>MCPTLNNIVSSLQRNGIFINSLIAALTIGGQQLFSSSTFSCPCQVGKNFYYGSAFLVIPALILLVAGFALRSQMWTITGEYCCSCAPPYRRISPLECKLACLRFFSITGRAVIAPLTWLAVTLLTGTYYECAASEFASVDHYPMFDNVSASKREEILAGFPCCRSAPSDVILVRDEIALLHRYQSQMLGWILITLAT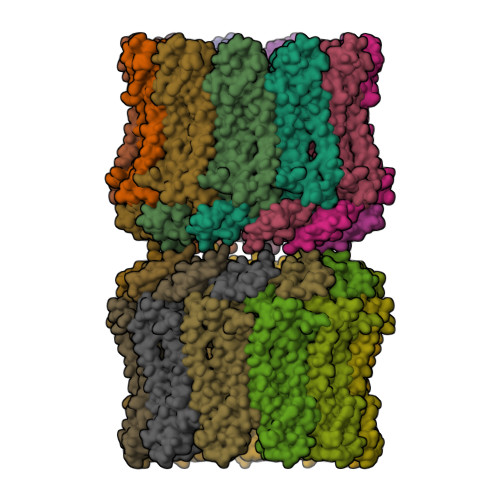IAALVSCCVAKCCSPLTSLQHCYWTSHLQNERELFEQAAEQHSRLLMMHRIKKLFGFIPGSEDVKHIRIPSCQDWKDISVPTLLCMGDDLQGHYSFLGNRVDEDNEEDRSRGIELKP[22x]>MKLFISPGACSLAPHIALRETGAAFDAVKVDLATRKVETGDDFLTVNPSGKVPALTLDSGETLTENPAILLYIADQKPDAALAPRDGTLERYRLISRLSFLGSEFHKAFVPLFTPGSSDEAKL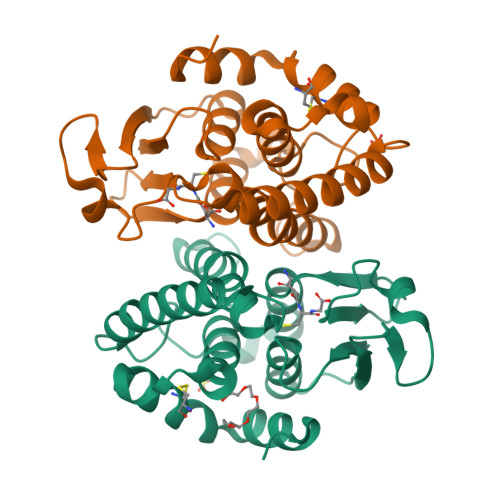AASTAVKNHLGALDKELLDKEHYAGSEFSVADIYLFVMLGWPAHVGIDMSAYPNLGAYCGRIAQRPSVGAALKAEGLV[2x]>RRLETQKEAEANRGYGKPSLGGPFHLEDMYGNEFTEKNLLGKFSIIYFGFSNCPDICPDELDKLGLWLNTLSSKYGITLQPLFITCDPARDSPAVLKEYLSDFHPSILGLTGTFDEVKNACKKYRVYFSTPPNVKPGQDYLVDHSIFFYLMDPEGQFVDALGRNYDEKTGVDKIVEHVKSY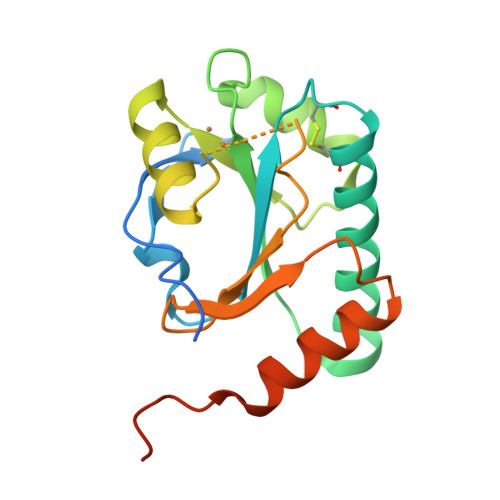VPAEQRAKQKEAWYSFLFK[4x]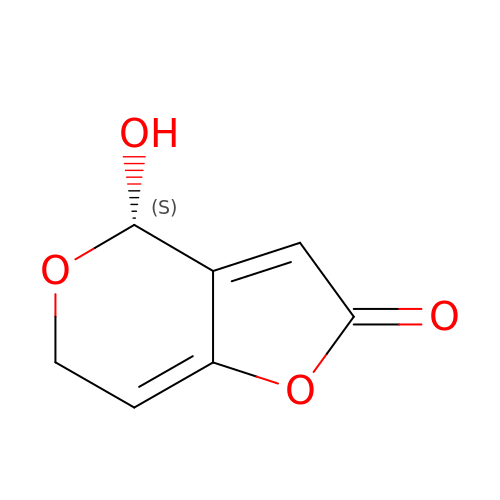(4~{S})-4-oxidanyl-4,6-dihydrofuro[3,2-c]pyran-2-one | C7 H6 O4 | ZRWPUFFVAOMMNM-ZETCQYMHSA-N> MFDGELIAKMVVELNAAMTSAQEALQFPDFEVVQKAQPTQQGTSTRPTIFFQKLFDIPRGWPATDWHLDNTTRKYVEITRQHVETTFQISSLHWQNPEITHVVTASDIANYVRAYFQARSTIERVKELDFLILRVSQISNEAFENDNHQFEFHPSFDMVVTYNQYIRLYENAAYS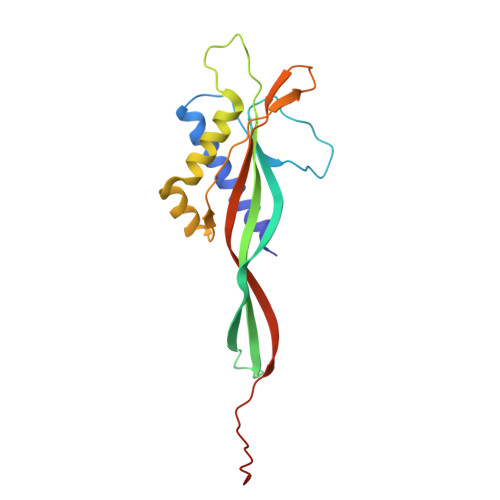ADGVLIGV> SFFFLSFHISNLQFNSSLEDPSTDYYQELQRDISEMFLQIYKQGGFLGLSNIKFRPG;> SVVVQLTLAFREGTINVHDVETQFNQYKTEAASRYNLTISDVSVSDVPFPFSA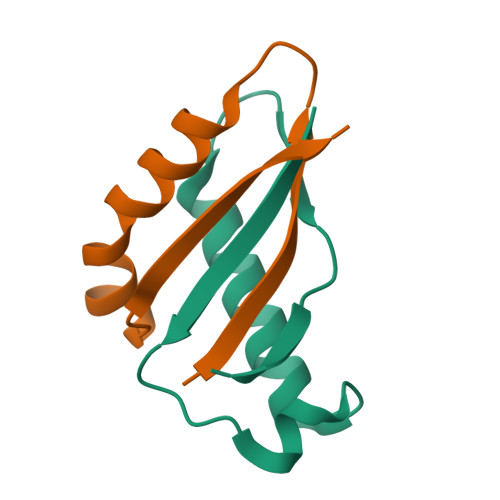QS> MFENITAT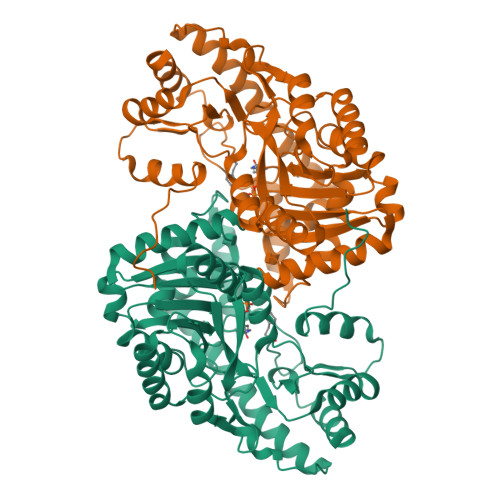TADPILGLADLFRADERPGKIDLGIGVYKDETGKTPVLTSVKKAEQYLLENETTKNYLGIDGIPEFGRCTQELLFGKGSALINDKRARTAQTPGGSGALRVAADFLAKNTSVKRVWVSNPSWPNHKSVFNSAGLEVREYAYYDAENHTLDFDALINSLNEAQAGDVVLFHGCCHNPTGIDPTLEQWQTLAQLSVEKGWLPLFDFAYQGFARGLEEDAEGLRAFAAMHKELIVASSYSKNFALYNERVGACTLVAADSETVDRAFGQMKAAIRANYSSPPAHGASVVATILSNDALRAIWEQELTDMRQRIQRMRQLFVNTLQEKGANRDFSFIIKQNGMFSFSGLTKEQVLRLREEFGVYAVASGRVNVAGMTPDNMAPLCEAIVAVL>[2x]GEIQWMRPSKEVGYPIINAPSKTKLEPSAFHYVFEGVKEPAVLTKNDPRLKTDFEEAIFSKYVGNKITEVDEYMKEAVDHYAGQLMSLDINTEQMCLEDAMYGTDGLEALDLSTSAGYPYVAMGKKKRDILNKQTRDTKEMQKLLDTYGINLPLVTYVKDELRSKT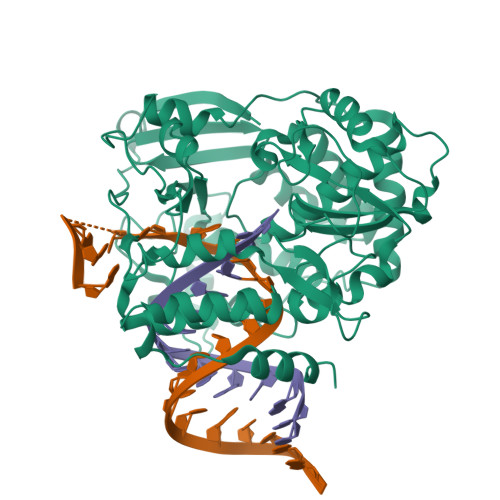KVEQGKSRLIEASSLNDSVAMRMAFGNLYAAFHKNPGVITGSAVGCDPDLFWSKIPVLMEEKLFAFDYTGYDASLSPAWFEALKMVLEKIGFGDRVDYIDYLNHSHHLYKNKTYCVKGGMPSGASGTSIFNSMINNLIIRTLLLKTYKGIDLDHLKMIAYGDDVIASYPHEVDASLLAQSGKDYGLTMTPADKSATFETVTWENVTFLKRFFRADEKYPFLIHPVMPMKEIHESIRWTKDPRNTQDHVRSLCLLAWHNGEEEYNKFLAKIRSVPIGRALDLPEYSTLYRRWLDSFGSSSHHHHHH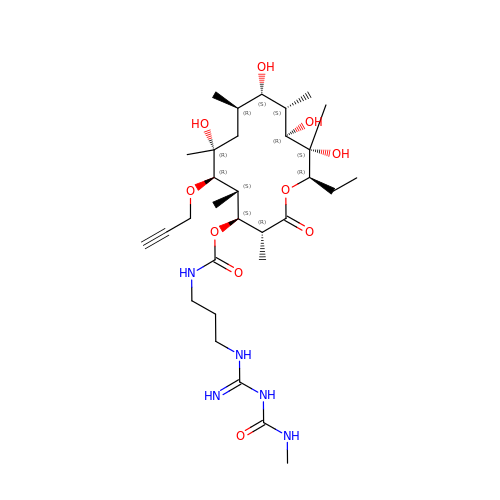(3R,4S,5S,6R,7R,9R,10S,11S,12R,13S,14R)-14-ethyl-7,10,12,13-tetrahydroxy-3,5,7,9,11,13-hexamethyl-2-oxo-6-(prop-2-yn-1-yloxy)oxacyclotetradecan-4-yl {3-[N'-(methylcarbamoyl)carbamimidamido]propyl}carbamate | C31 H55 N5 O10 | BOCNNNRHDZJQLM-BKUHWZEQSA-N> MA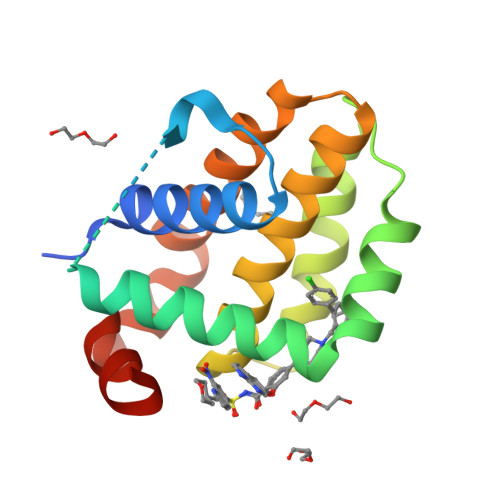HAGRTGYDNREIVMKYIHYKLSQRGYEWDAGDDVEENRTEAPEGTESEVVHLTLRQAGDDLSRRYRRDFAEMSSQLHLTPFTARGRFATVVEELFRDGVNWGRIVAFFEFGGVMCVESVNREMSPLVDNIALWMTEYLNRHLHTWIQDNGGWDAFVELYGPSMR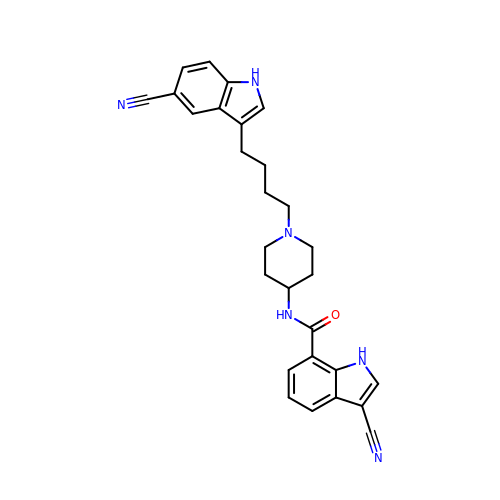3-cyano-N-{1-[4-(5-cyano-1H-indol-3-yl)butyl]piperidin-4-yl}-1H-indole-7-carboxamide | C28 H28 N6 O | GVZDPXYOJHKYRC-UHFFFAOYSA-N> TNVVPAKDAPTTNSPPSTTSPNQAAADANQQQAGIVSSQSGPNAVGDSAPSSSVNNDGDIITRPTSDSIAAVANATKPAAVVSDPQSMKVTPIVNPSSYVCNVCNARFSTMSALSEHLRSDHRDDASTLLATPMINNAIRSFLTAWDDIRILSPDVSSKSLSAYLDSAVANGPELIIEDTGLCTSFMLLDNIPSAHLTKELIGFTWFMQMYQMTPPLPEGAVNRIVCMTNWASLGDEGRGLEVRLPPPTDSSVHAYKTVLSRGYIDNAQFNPLALRSNVLLMLLQFTLSNLKINKSSTFTSDVTTITSGRMIRAFEGRPELLALAYPGRAVLPTQTKNAQFLSTAIADRIGRLDRANLIGGEVSAMVECMELCDALTLHIRETYIMLLRSMHQDPTQIVQIVNECANNLLNSTIPISLRPTILCPWFASSEDLRLQQVMHLVNISSNTAAALPLVEALSTLLRSVTPLVLDPTVLTNAITTISESTTQTISPISEILRLLQPMGNDYAAFWKCIASWAYNGLVTTVLSEDAFPDSSQSITHLPSMWKCLFLTLAGPMTSDPHSPVKVFMALANLLAQPEPIAIGVPGMHQTTPASQFSHPGVWPPGFLNPQLINPQQAPLLRAFAEHIRANWPQPSEFGYGSTLQGSANLFIPSNRMVYPWPNQPLPRLTVAPTYDSAMSNWISTTIAFFIRVVNSVNMTATVNDLTRRTMTGVMTAMRQVKTMTPFYIQHMCPTELSVLASVTVTPPFQVPFTRLVQNDVITNVLVARVDPAQRGDAAVDIRATHATFAAALPVDPAAIVVAMLCGQTETNLIPSHHYGKAFAPLFAS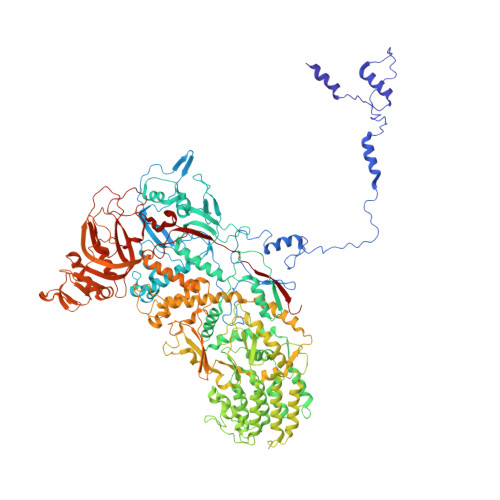NAMFTRNQRAVITREAFVCARSAVAQCQDAGFLVPRPLDALRQFDVTSAAAAEIMHAVNDAFKTAFDLDGALLDGLALYGDPRIADLSAAYLQYGGNVVREHVPPGPSHIHRALQQVESTFMAEMNLFNVARGNLYLVQTATNGNWSPMAPVAAPPFVRGGPNVRVVGRFGTIVPRPNGLEPQLIDDGNVPRDIAGDWVYPSDVLQVSVAVFRDYVWPMVKAGRTRVLVELGHYVYTLHYYDPQISLDEAPILEEWLSKINPAGIPPVPFCIPIPQVYPCITARRVHYAFTSENNNDSLFSTNAASIDTAFGENAAVSPLRWPGLVDPNYRVGTNDLPNRITLYNSLYRYNFTYPTLDGIMYVRSAT>MDLTVEPNLHSLITSTTHKWIFVGGKGGVGKTTSSCSIAIQMALSQPNKQFLLISTDPAHNLSDAFGEKFGKDARKVTGMNNLSCMEIDPSAALKDMNDMAVSRANNNGSDGQGDDLGSLLQGGALADLTGSIPGIDEALSFMEVMKHIKRQEQDEGETFDTVIFDTAPTGHTLRFLQLPNTLSKLLEKFGEITNKLGPMLNSFMGAGNVDISGKLNELKANVETIRQQFTDPDLTTFVCVCISEFLSLYETERLIQELISYDMDVNSIIVNQLLFAENDQEHNCKRCQARWKMQKKYLDQIDELYEDFHVVKMPLCA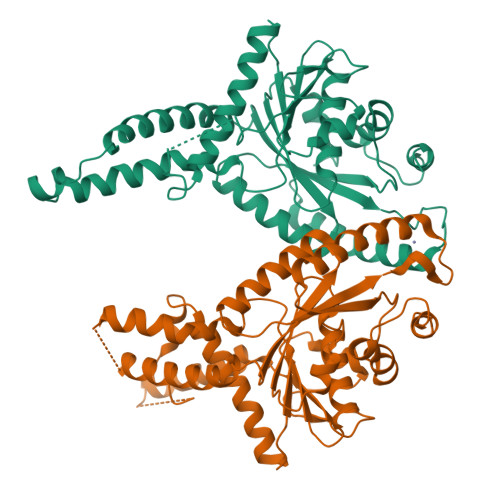GEIRGLNNLTKFSQFLNKEYNPITDGKVIYELEDKELEHHHHHH[2x]> ASRGSHHHHHHGASDDDDKEVVLLDFAAAGGELGWLTHPYGKGWDLMQNIMNDMPIYMYSVCNVMSGDQDNWLRTNWVYRGEAERIFIELKFTVRDCNSFPGGASSCKETFNLYYAESDLDYGTNFQKRLFTKIDTIAPDEITVSSDFEARHVKLNVEERSVGPLTRKGFYLAFQDIGACVA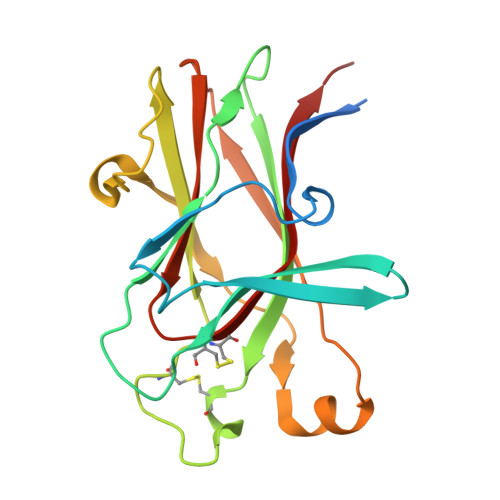LLSVRVYYKKC>MRLSWVIGGAQGTGIDTAANIFGNAVASAGYYIYGNREYYSNIKGRHSYFSLTISDKRVRSNTQKIDILVSFDAETVFQHFYDVKDILIYNKAVETTKIDAVQSMEPELAERIKDFLTKQGYETTVKGALEYASKNNVTLIPVNYDEIAKKVADEMKVPLSVTERVKNIVGITISYKLLGLDVNYLIEAINSTFKQDLYRKMNELAVKDSYDIVESRYNLKPSSKERRRFWLDGNTAVAIGKIYGGVRFQSYYPITPASDESVYIEAHQDVLMEDPITGDKKKGTIVVVQAEDELAAINMAIGAALTGVRAATATSGPGFSLMVEGLGWAGMNEVPVVITYYIRGGPSTGLPTRTAQSDLIFPIFAGHGEFPKIVLASGDHAEAFKDAIWALNLAEKYQTPVIHLVEKTLANSYSTIPYEELELDKLKAERGKIVESGDISYKRFKFTEDGISPRAFLGKATMYYTGDEHNEEGHISEDVVNRTMMYEKRMKKLEVADKEIPEESRVKIYGDLNSRNLIITWGSPTGVLRDILEESNFDFTLLQIRMFSPFPKNLVSKLMEGRDKIITVEGNYLAQTSLLVKMYTGKDVTNSILKWNGRPFLRDELEEALI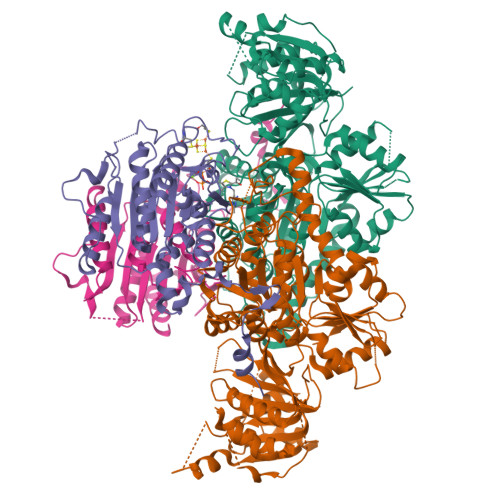KVIKDGEKRVVLNGGI[2x];>MAAFTPQWNDWCPGCGNFGILNAEQQAIVELGVDTKNVVVVSGIGCSGKIPHFFRTPISGVHTLHGRAIAFATGIKLSNPDLVVIVNGGDGDLLGIGAGHFVAAGRRNVDMVVILHDNGVYGLTKGQASPTLKRGEKPKSLPRPNINDAVNPIALAISSGYTFVARGYAYDVKHLKELIKSAIKHKGLALIDVLQPCPTYNDINTKEWYDKRIYKLDTLPDWDPVVKKPEEVNEKIKRAIDKSLEWGDRIPIGIFYQNELVPSYEERIKANSPAYLDYTPAKQLIEKEGKLTTIIDPLLKEREVD[2x]>MSLFNDKVAKLLAGHEALLMRKNEPVEEGNGVITRYRYPVLTAAHTPVFWRYDLNEETNPFLMERIGMNATLNAGAIKWDGKYLMLVRVEGADRKSFFAVAESPNGIDNFRFWEYPVTLPEDVVPATNVYDMRLTAHEDGWIYGIFCAERHDDNAPIGDLSSATATAGIARTKDLKNWERLPDLKTKSQQRNVVLHPEFVDGKYALYTRPQDGFIDTGSGGGIGWALIDDITHAEVGEEKIIDKRYYHTIKEVKNGEGPHPIKTPQGWLHLAHGVRNCAAGLRYVLYMYMTSLDDPTRLIASPAGYFMAPVGEERIGDVSNVLFSNGWIADDDGKVFIYYAS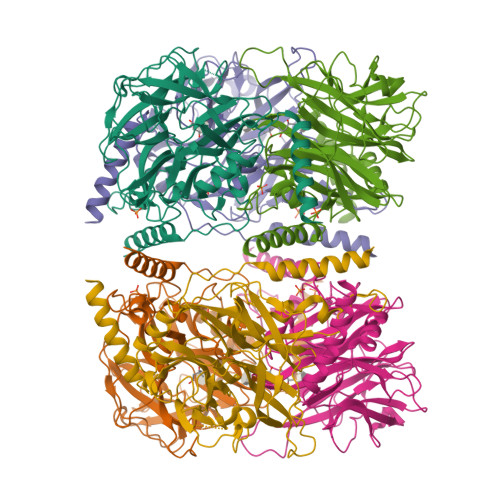SDTRMHVATSTIERLVDYCLHTPQDGFSSSASVEILKNLIERNLRLMK[2x]>[2x]MMAGPLSGLRVVELAGIGPGPHAAMILGDLGADVVRIDRPSSVDGISRDAMLRNRRIVTADLKSDQGLELALKLIAKADVLIEGYRPGVTERLGLGPEECAKVNDRLIYARMTGWGQTGPRSQQAGADINYISLNGILHAIGRGDERPVPPLNLVGDFGGGSMFLLVGILAALWERQSSGKGQVVDAAMVDGSSVLIQMMWAMRATGMWTDTRGANMLDGGAPYYDTYECADGRYVAVGAIEPQFYAAMLAGLGLDAAELPPQNDRARWPELRALLTEAFASHDRDHWGAVFANSDACVTPVLAFGEVHNEPHIIERNTFYEANGGWQPMPAPRFSRTASSQPRPPAATIDIEAVLTDWDGGSGC

α-Methylacyl-CoA racemase in M. tuberculosis (MCR) has an essential role in fatty acid metabolism and cholesterol utilization, contributing to the bacterium’s survival and persistence. It catalyses the racemization of α-methyl-branched fatty acyl-CoAs, converting the (2S)-epimer to a near racemic mixture of the (2R)- and (2S)-epimers. The enzyme enables the conversion of α-methyl-branched fatty acids derived from cholesterol metabolism into forms that can be utilized by M. tuberculosis for growth and persistence within the host, a key component of M. tuberculosis pathogenesis. Within each active site, the large domain contributes the catalytic residues H126 (part of α-helix 3) and D156 (part of α-helix 5), while the small domain contributes a third catalytic residue, E241 (part of α-helix 9).

Crystals of the three MCR mutants H126A, D156A and E241A were obtained using identical conditions to those used with the wild-type enzyme and diffracted to 2.45, 1.64 and 1.85 Å resolutions, respectively. The three mutants collectively had fewer hydrogen bond interactions; within the H126A, D156A and E241A mutants, 3, 5 and 5 interactions were observed, respectively. The active site of the H126A mutant underwent the most profound structural change due to the loss of the imidazole ring, although D156 and its hydrogen bond interactions remained unaffected. The E241 side-chain which is hydrogen-bonded to H126 within the wild-type, is rotated by around 90° and projects away from the active site due to loss of its binding partner (H126). Interestingly, the normalized temperature factor (B-value, 45.79 Å2) of this E241 side-chain is lower than expected due to the peripheral Q243 (39.70 Å2) residue hydrogen bonding to it. As the E241 residue is stabilized by Q243, it moves away from D156, and hence, it cannot substitute the central structural role of the imidazole ring of H126. Consequently, five H126-mediated hydrogen bond interactions are lost. The observed displacement of E241 also suggests that it is unlikely to substitute the catalytic function of H126, which implies that the residual enzymatic activity observed in the H126A mutant is facilitated solely by the D156 side-chain. Wild-type MCR was the most efficient enzyme with a kcat/Km of 1.07 × 106 M−1.s−1, while the H126A mutant was the least efficient at 0.11 × 106 M−1.s−1. This near 10-fold decrease in catalytic efficiency for the H126A mutant relative to wild-type MCR contrasts with the near abolition of activity previously observed, but shows that although all three mutants had diminished activity, the H126A mutation was most detrimental.> MKKYKYIAVCLMASVLLTTGCADSFLEVSSPTDETIDTYFTTDEHIQEAVVAAYDPLHWPDWAFDEYNPVNLMSDIMADDLWVGGDSKTDNQPWHLMMNFEAIPTNMIYG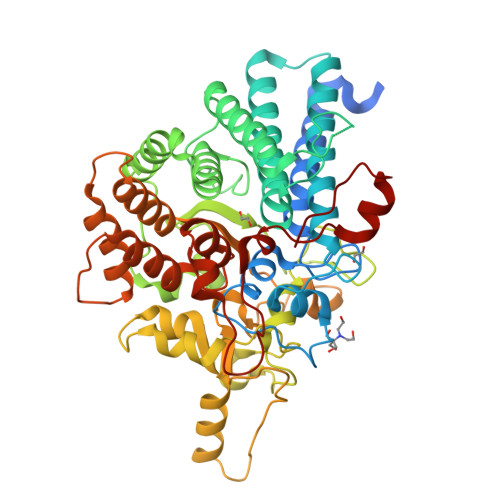LWKCAYSGVKRCNDVITYLDWATDVTDANRAYYEAQVIALRVFYYNWVWKFWGNVPYFDKNLTAPYVAEQLTADQLYEKMVTSLEEVIQLNVLPMREDSENYGRVTLAMVYMLYAEIVMYQNDDSRYSTALKYMEEIISSPQYDLMPDYTDIFKETGEWSIESIFEINYKDDNAVRDWGSPLVAGGTALPTLISPYIWPNGTDNHDRGWGFCPVRKETYERYSNNDTRRNATCWNAQAVLDAHNAEHPGDKLSYTTRYQDTGFFLEKYAAITGNNKDQKSSSELNWNNNLRIYRYSETLLNAAELITRGAGQGDAKKYLNLVHKRAGLVTEIEPTLDNIIEERHLEFVGEGKRYWDLIRTGKAASVLVPDAYGYRTNSWSSSKKYLPIPQKEIDAAKGTLVQNNY>MSKKEININNYNDDAIQVLEGLDAVRKRPGMYIGSTDGAGLHHLVWEIVDNAVDEALSGFGDRIDVTINKDGSLTVQDHGRGMPTGMHAMGIPTVEVIFTILHAGGKFGQGGYKTSGGLHGVGSSVVNALSSWLEVEITRDGAVYKQRFENGGKPVTTLKKIGTAPKSKTGTKVTFMPDATIFSTTDFKYNTISERLNESAFLLKNVTLSLTDKRTDEAIEFHYENGVQDFVSYLNEDKEILTPVLYFEGEDNGFQVEVALQYNDGFSDNILSFVNNVRTKDGGTHETGLKSAITKVMNDYARKTGLLKEKDKNLEGSDYREGLAAVLSILVPEEHLQFEGQTKDKLGSPLARPVVDGIVADKLTFFLMENGELASNLIRKAIKARDAREAARKARDESRNGKKNKKDKGLLSGKLTPAQSKNPAKNELYLVEGDSAGGSAKQGRDRKFQAILPLRGKVINTAKAKMADILKNEEINTMIYTIGAGVGADFSIEDANYDKIIIMTDADTDGAHIQTLLLTFFYRYMRPLVEAGHVYIALPPLYKMSKGKGKKEEVAYAWTDGELEELRKQFGKGATLQRYKGLGEMNADQLWETTMNPETRTLIRVTIEDLARAERRVNVLMGDKVEPRRKWIEDNVKFTLEEATVFHMSNIQNMSLEDIMGERFGRYSKYIIQDRALPDIRDGLKPVQRRILYSMNKDSNTFDKSYRKSAKSVGNIMGNFHPHGDSSIYDAMVRMSQNWKNREILVEMHGNNGSMDGDPPAAMRYTEARLSEIAGYLLQDIEKKTVPFAWNFDDTEKEPTVLPAAFPNLLVNGSTGISAGYATDIPPHNLAEVIDAAVYMIDHPTAKIDKLMEFLPGPDFPTGA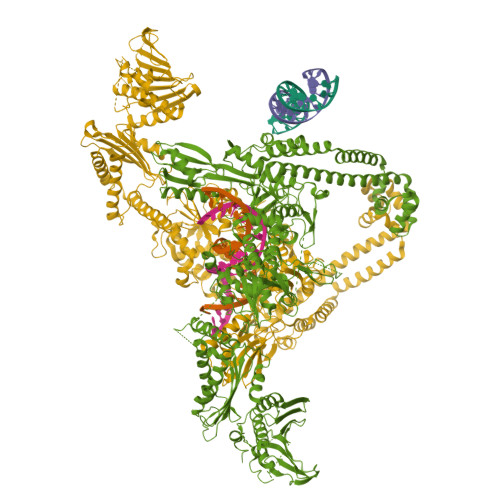IIQGRDEIKKAYETGKGRVVVRSKTEIEKLKGGKEQIVITEIPYEINKANLVKKIDDVRVNNKVAGIAEVRDESDRDGLRIAIELKKDANTELVLNYLFKYTDLQINYNFNMVAIDNFTPRQVGIVPILSSYIAHRREVILARSRFDKEKAEKRLHIVEGLIRVISILDEVIALIRASENKADAKENLKVSYDFTEEQAEAIVTLQLYRLTNTDVVVLQEEEAELREKIAMLAAIIGDERTMYNLMKKELREVKKKFATPRLSSLEDTAKALEHHHHHH[2x]>QSITDYNYKKPLHNDYQILDKSKIFGSNSGSFVMYSMAADAYYIYNEKESRKRYSPNSTYKIYLAMFGLDRHIINDENSRMSWNHKHYPFDAWNKEQDLNTAMQNSVNWYFERISDQIPKNYTATQLKQLNYGNKNLGSYKSYWMEDSLKISNLEQVIVFKNMMEQNNHFSKKAKNQLSSSLLIKKNEKYELYGKTGTGIVNGKYNNGWFVGYV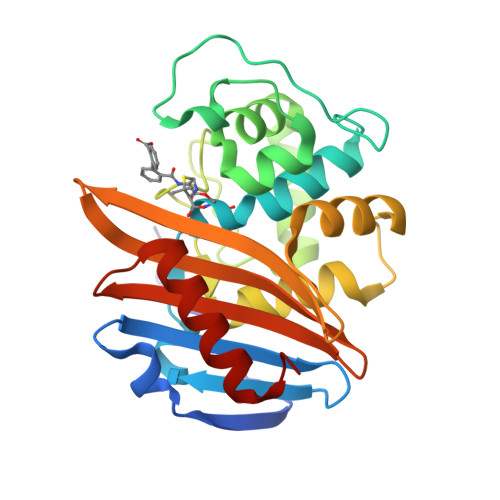ITNHDKYYFATHLSDGKPSGKNAELISEKILKEMGVLN[2x]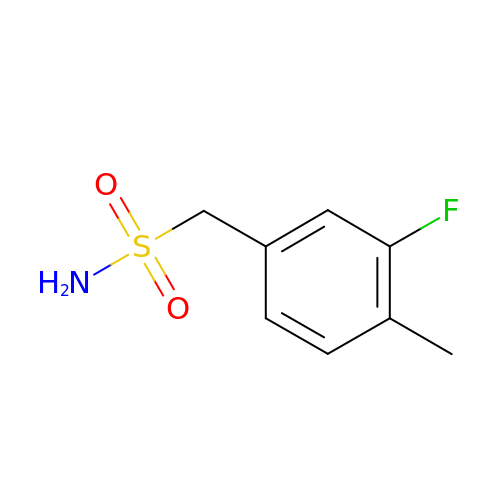1-(3-fluoro-4-methylphenyl)methanesulfonamide | C8 H10 F N O2 S | BRGBJOARAPZJCN-UHFFFAOYSA-N>GSAMASNAVLYKSNHNVVYSCKYHIVWCPKYRRKVLVGAVEMRLKEIIQEVAKELRVEIIEMQTDKDHIHILADIDPSFGVMKFIKTAKGRSSRILRQEFNHLKTKLPTLWTNSCFISTVGGAPLNVVKQYIENQQNSNRPKQKEKWKSYVDNLQTKAL[4x]

One of the simplest and best characterized TEs is the bacterial insertion sequence (IS) IS608 from Helicobacter pylori, a member of the IS200/IS605 family. It exhibits an unusual transposition mechanism using single-stranded DNA (ssDNA) intermediates and integrates specifically at 4 nt target sequences in the genome. Transposon excision and integration is catalyzed by the IS608-encoded transposase TnpA, which belongs to the HUH (histidine–hydrophobic–histidine) endonuclease superfamily and uses a single catalytic tyrosine to cleave DNA. Previous crystallographic and biochemical studies of IS608 have shown that TnpA binds specifically to sub-terminal imperfect palindrome (IP) structures formed on the top strand of the left (LE) and right (RE) IS ends (named IPL and IPR, respectively). Its catalytic site is assembled in trans within a protein dimer, with the catalytic tyrosine (located on the most C-terminal helix αD) contributed by one monomer and the HUH motif by the other.

In this work, we determined the crystal structure of IS608 TnpA in complex with a 29-mer LE (LE29) and a 6-mer target oligo (T6’) at 2.6 Å resolution. LE29 includes a 3 nt extension at the 3′ base of IPL (positions +42 to +44) and T6’ represents uncleaved target DNA with a cytosine base at position +1 downstream of the cleavage site. In order to trap the active pre-cleavage state of the complex, crystals with wild type TnpA were grown in the presence of Ca2+. The asymmetric unit of the TnpA/LE29/T6’ crystals contains two copies of a ternary complex, each consisting of a TnpA dimer bound to two LE and two target DNA molecules. As previously observed in the TnpA/LE26/T6 complex, A+16 and A+17 in LE29 GL form base pairs with target bases T−3 and T−4, respectively. However, in our structure these pairs also interact with T+43 and A+42 at the 3′ base of IPL, together assembling a set of two base triplets. In the fourth T6’ molecule, C+1 points towards the A+18 base in LE29 and it is stabilized by π-stacking interactions with Y7 (chain B) and F112 (chain A). In this case, C+1 occupies the position that was occupied by the catalytic Y127 in the previously described TnpA/LE26/T6 structure, and helix αD (carrying Y127, chain B) has moved closer to the active site where it is stabilized by hydrophobic contacts and hydrogen bonds involving Q132 and K125 in αD with Q59, E37 and E57 in the protein core, respectively. In this conformation, Y127 is placed in a cleavage-competent position, such that its nucleophile hydroxyl group is positioned 3.0 Å from the phosphorous atom of the scissile phosphate in C+1. The Ca2+ ion is coordinated by H64 and H66 (β4, chain A), D61 (β3, chain A), Q131 (αD, chain B), C−1/O3′ (target DNA), a water molecule and potentially the scissile phosphate (C+1/OP1, target DNA).(9R,11S)-3-ethyl-11-[(1R)-1-hydroxy-2-({[3-(propan-2-yl)phenyl]methyl}amino)ethyl]-9-methyl-3,12-diazabicyclo[12.3.1]octadeca-1(18),14,16-triene-2,13-dione | C31 H45 N3 O3 | 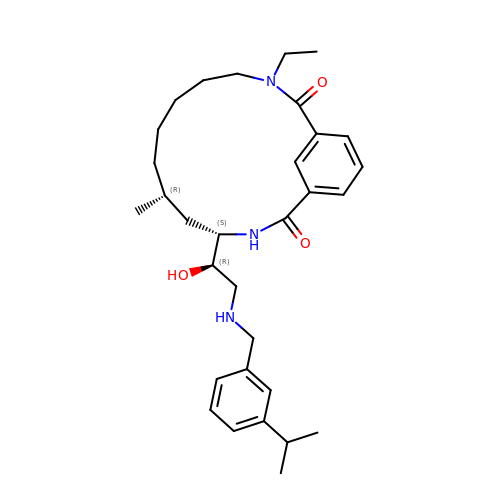MYMHIVTZLXPTIU-LDVROUIZSA-N>[2x]MDLPPDSRTALRDWLTEQLADLLGEPLADVRALADDDDLLGCGLDSIRLMYLQERLRARGSTLDFAQLAQRPCLGAWLDLLACADRLSAPATVALPTAQDRDQPFELSSVQQAYWLGRGAGEVLGNVSCHAFLEFRTRDVDPQRLAAAAECVRQRHPMLRARFLDGRQQILPTPPLSCFDLQDWRTLQVDEAERDWQALRDWRAHECLAVERGQVFLLGLVRMPGGEDRLWLSLDLLAADVESLRLLLAELGVAYLAPERLAEPPALHFADYLAHRAAQRAEAAARARDYWLERLPRLPDAPALPLACAPESIRQPRTRRLAFQLSAGESRRLERLAAQHGVTLSSVFGCAFALVLARWSESAEFLLNVPLFDRHADDPRIGEVIADFTTLLLLECRMQAGVSFAEAVKSFQRNLHGAIDHAAFPALEVLREARRQGQPRSAPVVFASNLGEEGFVPAAFRDAFGDLHDMLSQTPQVWLDHQLYRVGDGILLAWDSVVGLFPEGLPETMFEAYVGLLQRLCDSAWGQPA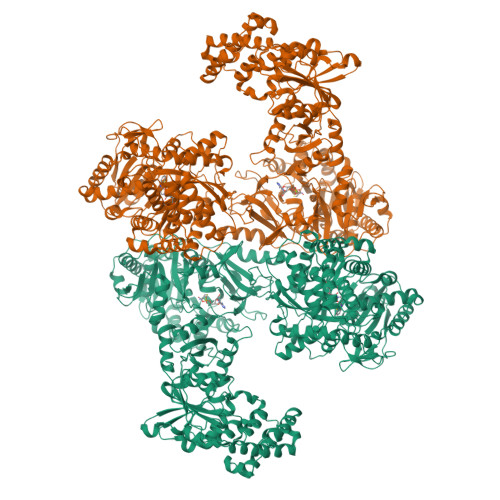DLPLPWAQQARRALLNGQPACATARTLHRDFFLRAAEAPDADALLYRDQRVTRGELAERALRIAGGLREAGVRPGDAVEVSLPRGPQQVAAVFGVLAAGACYVPLDIDQPPARRRLIEEAAGVCLAITEEDDPQALPPRLDVQRLLRGPALAAPVPLAPQASAYVIYTSGSTGVPKGVEVSHAAAINTIDALLDLLRVNASDRLLAVSALDFDLSVFDLFGGLGAGASLVLPAQEQARDAAAWAEAIQRHAVSLWNSAPALLEMALSLPASQADYRSLRAVLLSGDWVALDLPGRLRPRCAEGCRLHVLGGATEAGIWSNLQSVDTVPPHWRSIPYGRPLPGQAYRVVDTHGRDVPDLVVGELWIGGASLARGYRNDPELSARRFVHDAQGRWYRTGDRGRYWGDGTLEFLGRVDQQVKVRGQRIELGEVEAALCAQAGVESACAAVLGGGVASLGAVLVPRLAPRAEGSMDLPAAQPFAGLAEAEAVLTREILGALLEAPLELDDGLRRRWLDWLADSAASALPSLDEALRRLGWQAAGLTAMGNALRGLLAGEQAPAALLLDPWLAPQAVAARLPDGREALARLLEALPTPAAGERLRVAVLDTRAGLWLDQGMASLLRPGLELTLFERSRVLLDAAATRLPERIVVQALDDGLLPAEHLGRYDRVISFAALHAYEASREGLALAAALLRPQGRLLLVDLLCESPLALLGAALLDDRPLRLAELPSLLADLAAAGLAPRCLWRSERIALVEALAPGLGLDAAALQAGLEQRLPQAMRPERLWCLPSLPLNGNGKVDRRRLAESMTRALGECRHEPSAEEPLEAHEQALAECWEAVLKRPVRRREASFFSLGGDSLLATRLLAGIRERFGVRLGMADFYRQPTLAGLARHLQVQTVEIEETQLEEGVLHHHHHHLPSWSHPQFEK(1S,2S,3S,4R,5R)-2-amino-4-[(2S)-2-(hydroxymethyl)pyrrolidin-1-yl]-6,8-dioxabicyclo[3.2.1]octan-3-ol 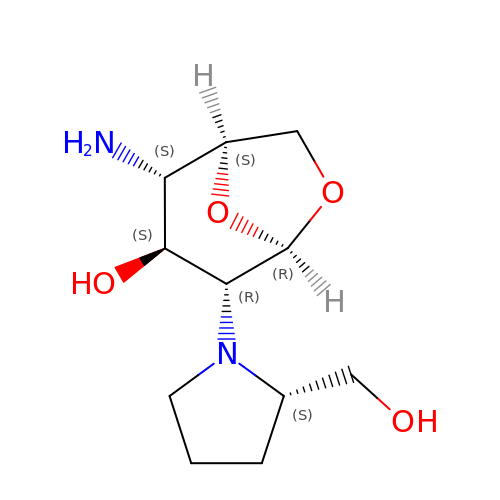| C11 H20 N2 O4 | NMTUCAAUKBQRDV-ZESFFYIMSA-N>[2x]GPHMLEHSGISQASEYDDPPGLREKAEYLLREWVNLYHSAAAGRDSTKAFSAFVGQMHQQGILKTDDLITRFFRLCTEMCVEISYRAQAEQQHNPAANPTMIRAKCYHNLDAFVRLIALLVKHSGEATNTVTKINLLNKVLGIVVGVLLQDHDVRQSEFQQLPYHRIFIMLLLELNAPEHVLETINFQTLTAFCNTFHILRPTKAPGFVYAWLELISHRIFIARMLAHTPQQKGWPMYAQLLIDLFKYLAPFLRNVELTKPMQILYKGTLRVLLVLLHDFPEFLCDYHYGFCDVIPPNCIQLRNLILSAFPRNMRLPDPFTPNLKVDMLSEINIAPRILTNFTGVMPPQFKKDLDSYLKTRSPVTFLSDLRSNLQVSNEPGNRYNLQLINALVLYVGTQAIAHIHNKGSTPSMSTITHSAHMDIFQNLAVDLD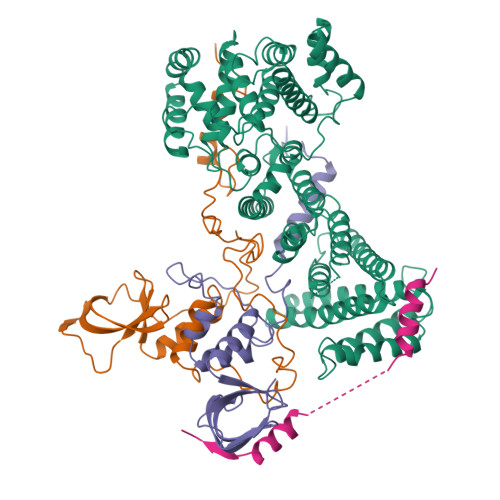TEGRYLFLNAIANQLRYPNSHTHYFSCTMLYLFAEANTEAIQEQITRVLLERLIVNRPHPWGLLITFIELIKNPAFKFWNHEFVEEEPEIEKLFQSVAQCCM;>GPHMLEMVTDQFGMIGLLTFIRAAETDPGMVHLALGSDLTTLGLNLNSPENLYPKFASPWASSPCRPQDIDFHVPSEYLTNIHIRDKLAAIKLGRYGEDLLFYLYYMNGGDVLQLLAAVELFNRDWRYHKEERVWITRAPGMEPTMKTNTYERGTYYFFDCLNWRKVAKEFHLEYDKLEERPHLPSTFNYNPAQQAF[2x];>GPHMLELTKEQLYQQAMEEAAWHHMPHPSDSERIRQYLPRNPCPTPPYHHQMPPPHSDTVEFYQRLSTETLFFIFYYLEGTKAQYLAAKALKKQSWRFHTKYMMWFQRHEEPKTITDEFEQGTYIYFDYEKWGQRKKEGFTFEYRYLE[2x];>GPHMLESHQQTDEIARSLKIFAQVTTGAAENAAGSMQDVMQEFATNGYASDDLG[2x]The transformation of UDP-D-GlcNAc in UDP-L-FucNAc requires three enzymes (CapE, CapF and CapG) in S. aureus. The two reactions catalysed by CapE are the C-4/C-6 dehydration and the C-5 epimerization of the UDP–sugar. CapE consists of three well-defined regions: a Rossmann domain for binding the coenzyme NADPH, a substrate binding domain, and a 23-residue loop peripheral to the protein core. Herein we present the first crystal structure of CapE, revealing that this enzyme forms a stable and functional homo-hexamer.

The third structure corresponds to wild-type protein (coenzyme-free) in complex with the substrate analogue UDP-6N3-GlcNAc. The substrate-analogue UDP-6N3-GlcNAc is clearly visible in the electron density map. The electron density of the azide moiety is weaker than that in other sections of the substrate analogue, probably because of radiation damage at this functional group. Although the sugar ring of the substrate analogue protrudes into the coenzyme domain (where the active site is located), it occupies a non-catalytic conformation compared with that of other representative SDR enzymes. The conformation of UDP-6N3-GlcNAc bound to CapE is similar to that of the inhibitor UDP-D-GalNAc bound to the homologous enzyme FlaA1. In particular, the UDP moiety of the substrate analogue establishes numerous H-bond and electrostatic interactions with polar residues of the protein. Unexpectedly, the coenzyme moiety is not observed in the structure of CapE in complex with substrate analogue. The latch is not observed in the two crystal structures of CapE with coenzyme bound because of dynamic disorder. In contrast, the latch is clearly observed in the structure with substrate analogue bound (see below). The analysis with DYNDOM indicates that the substrate-binding domain rotates 11° and moves a few angstroms towards the coenzyme-binding domain upon exit of the coenzyme and binding of substrate analogue. The latch is a flexible element that increases the contact surface area of adjacent monomers of CapE in the presence of the substrate analogue UDP-6N3-GlcNAc.

>MNHKHHHHHHSSGLVPRGSAMGFDDKILLITGGTGSFGNAVMKRFLDSNIKEIRIFSRDEKKQDDIRKKYNNSKLKFYIGDVRDSQSVETAMRDVDYVFHAAALKQVPSCEFFPVEAVKTNIIGTENVLQSAIHQNVKKVICLSTDKAAYPINAMGISKAMMEKVFVAKSRNIRSEQTLICGTRYGNVMASRGSVIPLFIDKIKAGEPLTITDPDMTRFLMSLEDAVELVVHAFKHAETGDIMVQKAPSSTVGDLATALLELFEADNAIEIIGTRHGEKKAETLLTREEYAQCEDMGDYFRVPADSRDLNYSNYVETGNEKITQSYEYNSDNTHILTVEEIKEKLLTLEYVRNELNDYKASMR[2x]>MAPSMIPFTIKLKTCLKMCIQRLRYAQEKQQAIAKQSRRQVAQLLLTNKEQKAHYRVETLIHDDIHIELLEILELYCELLLARVQVINDISTEEQLVKEHMDDGINEAIRSLIYAILFVDEVKELSQLKDLMAWKINVEFVNGVIADHIDVPEKIIKKCSPSVPKEELVDLYLKEIAKTYDVPYSKLENSLSS[2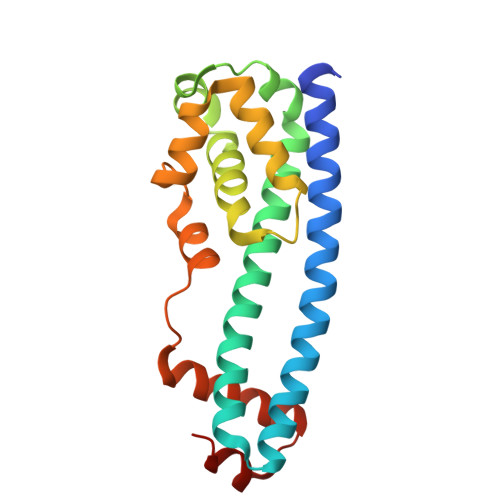x]>GSHMALAEKFNLQDRFLNHLRVNKIEVKVYLVNGFQTKGFIRSFDSYTVLLESGNQQSLIYKHAIST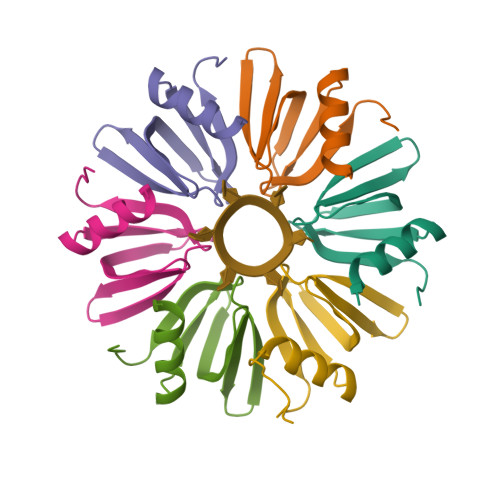IIPSSYVMLMPKKQETAQEAETSENEGS[12x]>[2x]MDGFSRRRMLMTGGALGAVGALGAATRALARPLWTWSPSASVAGTGVGVDPEYVWDEEADPVLAAVIDRGEVPAVNALLKQWTR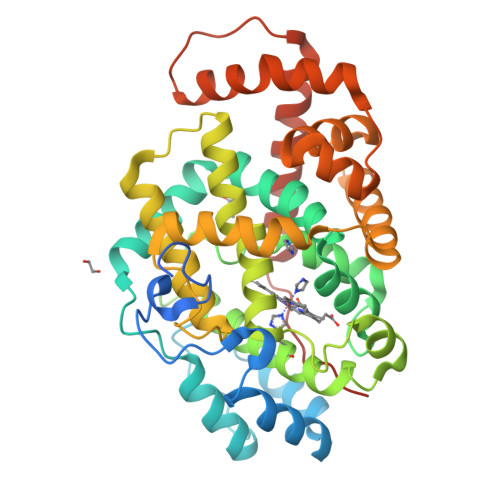NDQALPGGLPGDLREFMEHARRMPSWADKAALDRGAQFSKTKGIYVGALYGLGSGLMSTAIPRESRAVYYSKGGADMKDRIAKTARLGYDIGDLDAYLPHGSMIVTAVKTRMVHAAVRHLLPQSPAWSQTSGGQKIPISQADIMVTWHSLATFVMRKMKQWGVRVNTADAEAYLHVWQVSAHMLGVSDEYIPATWDAANAQSKQVLDPILAHTPEGEALTEVLLGIVAELDAGLTRPLIGAFSRYTLGGEVGDMIGLAKQPVLERLIATAWPLLVAFREGLIPLPAVPAVLWTLEEALRKFVLLFLSEGRRIAIDIPDVNRPS> MKTPALPTVQSPLLSSLPGVKHAFFTRQGGVSKGIYDSLNVGR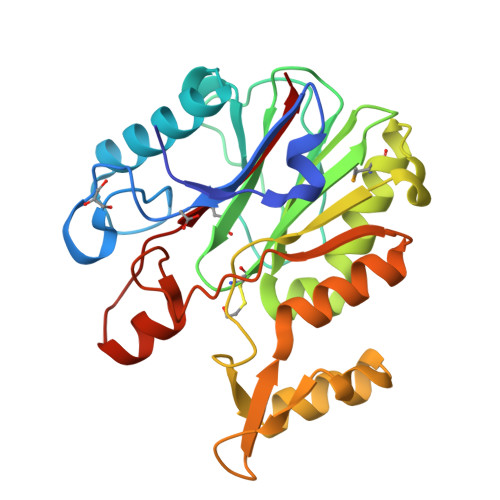GSQDEPADVEENRARIARWFGGGPEDLNVCYQIHSTIAIVADGSWGDARPEGDAVVSKTPGVICGAMAADCAPVLLVDPEARIVAAAHAGWRGALDGVVQSAVDRMVELGASPANITGVVGPCIGPKSYEVGLEFLHRFEADCPGSGRFFKPGASEDKRFFDLPAFVLDRLATAGVERREWVGRDTRAEEEWFFSNRRAFLNNDGDYGRLLSAITLEA> RSAFSKIESEEYNSLKSSTIQTIGTSDGGSGIGYIESGDYLVFNKINFGNGANSFKARVASGADTPTNIQLRLGSPT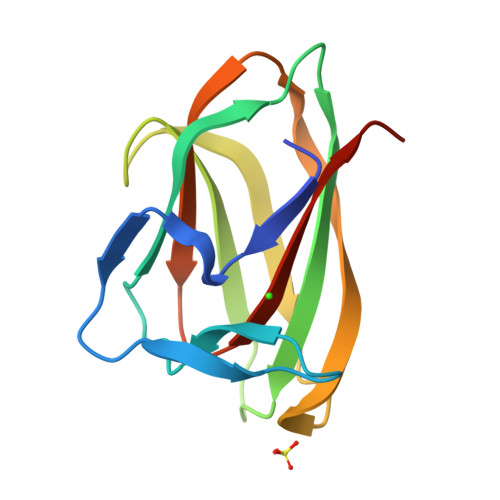GTLIGTLTVASTGGWNNYEEKSCSITNTTGQHDLYLVFSGPVNIDYFIFDSNGVNP> MAGKLPIVGEVVLPILRGHEDLSNPISTV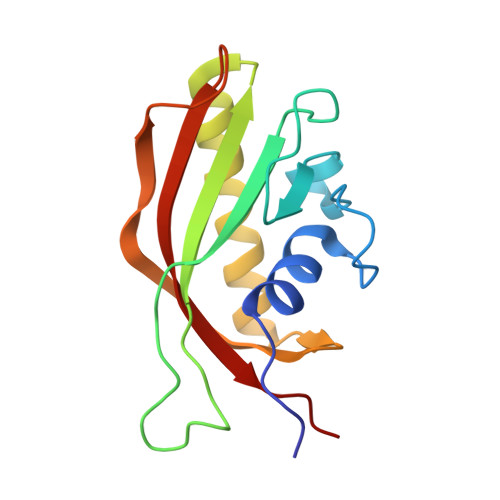PSLAGVHVGTWVEDIDSRTFPLITVRRVGGTRSPEHPTLFTQPVVEMTAYSAADLPTTEQMYEDALEVLYRAARLQTKTPAGYLHSVTETLGASHGPSPFDRTWRVFGLIRLGIRPPKN>MASSINNRKPSEIFKAQALLYKNMYAFVDSMSLKWSIEMNIPNIIHNHGKPITLSNLVSILQIPSTKVDNVQRLMRYLAHNGFFEIITNQELENEEEAYALTVASELLVKGTELCLAPMVECVLDPTLSTSFHNLKKWVYEEDLTLFAVNLGCDLWEFLNKNPEYNTLYNDALASDSKMINLAMKDCNLVFEGLESIVDVGGGNGTTGKIICETFPKLTCVVFDRPKVVENLCGSNNLTYVGGDMFISVPKADAVLLKAVLHDWTDKDCIKILKKCKEAVTSDGKRGKVIVIDMVINEKKDENQLTQIKLLMNVTISCVNGKERNEEEWK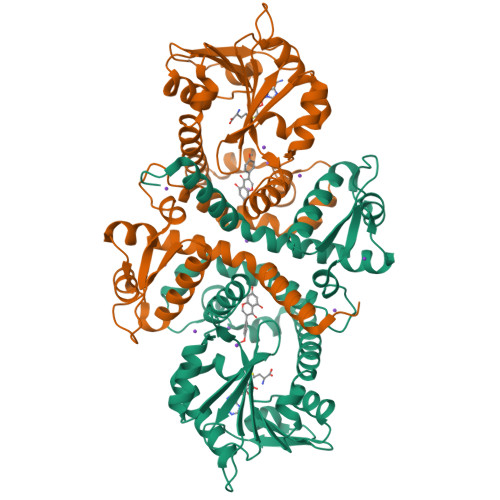KLFIEAGFQDYKISPFTGLMSLIEIYP[2x]>MNQLNTAIVEKEVIDPMAFRRALGNFATGVTIMTAQTSSGERVGVTANSFNSVSLDPALVLWSIDKKSSSYRIFEEATHFGVNILSAAQIELSNRFARRSEDKFANIEFDLGVGNIPLFKNCSAAFECERYNIVEGGDHWIIIGRVVKFHDHGRSPLLYHQGAYSAVLP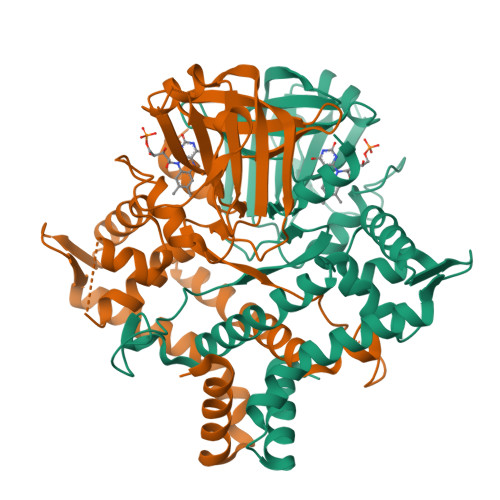HPSLNMKSETAEGVFPGRLYDNMYYLLTQAVRAYQNDYQPKQLASGFRTSEARLLLVLESKTASSKCDLQREVAMPIREIEEATKILSEKGLLIDNGQHYELTEQGNACAHMLYKIAESHQEEVFAKYTVDERKLFKNMLKDLIGI[2x]> MANKGRLGEQEAFAMTVPLLIDVDSSQQEALEAIALNDELVRVRRALYLDLGVPFP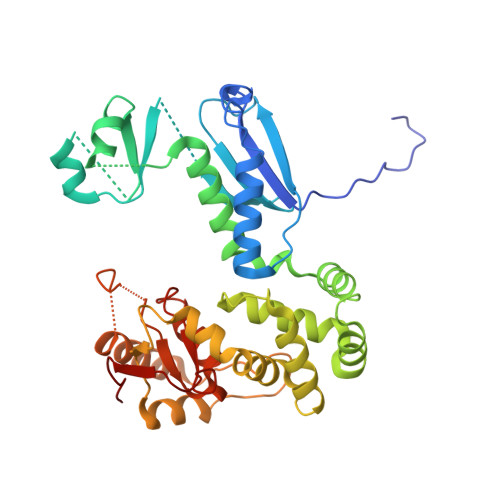GIHLRFNEGMGEGEYLISLQEVPVARGELKAGYLLVRESVSQLELLGIPYEKGEHLLPDQETFWVSVEYEERLEKSQLEFFSHSQVLTWHLSHVLREYAEDFIGIQETRYLLEQMEGGYGELIKEVQRIVPLQRMTEILQRLVGEDISIRNMRSILEAMVEWGQKEKDVVQLTEYIRSSLKRYICYKYANGNNILPAYLFDQEVEEKIRSRVRQTSAGSYLALDPAVTESLLEQVRKTIGDLSQIQSKPVLIVSMDIRRYVRKLIESEYYGLPVLSYQELTQQINIQPLGRVCL2-((4-acetyl-3-cyclopropyl-3,4-dihydroquinoxalin-1(2H)-yl)methyl)benzoic acid 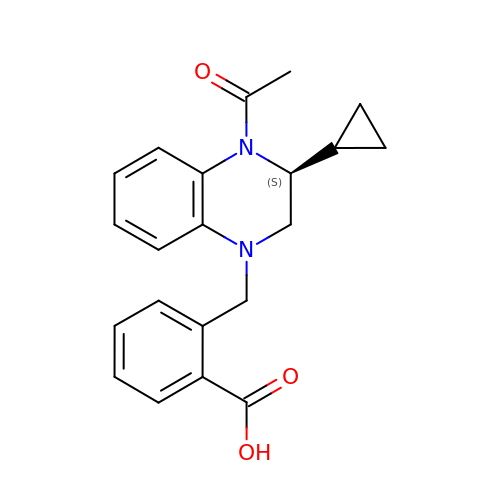| C21 H22 N2 O3 | PPKDQAUERJXIAY-HXUWFJFHSA-N> GPLGSPLTASMLASAPP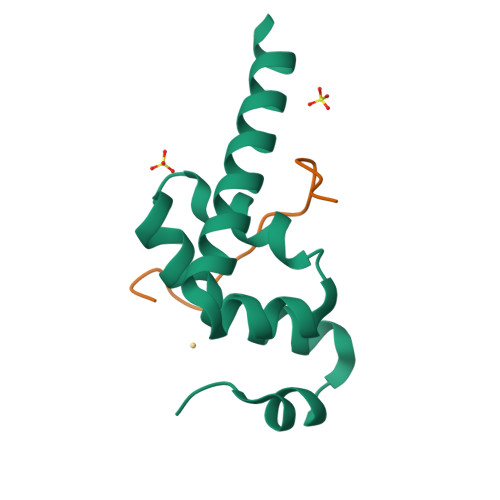QEQKQMLGERLFPLIQAMHPTLAGKITGMLLEIDNSELLHMLESPESLRSKVDEAVAVLQAHQAKEAAQKA;> STLNPNAKEFNPRSFSQ> GAAU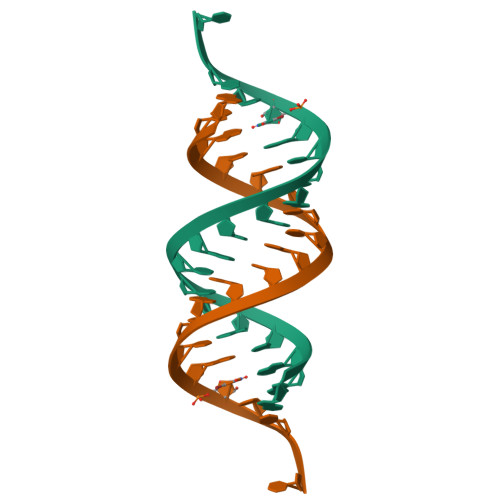GCCUGCGAGCAUCCC> MKIQMRNKKVLSFLTLTAIVSQALVYPVYAQTSTSNHSNKKKEIVNEDILPNNGLMGYYFTDEHFKDLKLMAPIKDGNLKFEEKKVDKLLDKDKSDVKSIRWTGRIIPSKDGEYTLSTDRDDVLMQVNTESTISNTLKVNMKKGKEYKVRIELQDKNLGSIDNLSSPNLYWELDGMKKIIPEENLFLRDYSNIEKDDPFIPNNNFFDPKLMSDWEDEDLDTDNDNIPDSYERNGYTIKDLIAVKWEDSFAEQGYKKYVSNYLESNTAGDPYTDYEKASGSFDKAIKTEARDPLVAAYPIVGVGMEKLIISTNEHASTDQGKTVSRATTNSKTESNTAGVSVNVGYQNGFTANVTTNYSHTTDNSTAVQDSNGESWNTGLSINKGESAYINANVRYYNTGTAPMYKVTPTTNLVLDGDTLSTIKAQENQIGNNLSPGDTYPKKGLSPLALNTMDQFSSRLIPINYDQLKKLDAGKQIKLETTQVSGNFGTKNSSGQIVTEGNSWSDYISQIDSISASIILDTENESYERRVTAKNLQDPEDKTPELTIGEAIEKAFGATKKDGLLYFNDIPIDESCVELIFDDNTANKIKDSLKTLSDKKIYNVKLERGMNILIKTPTYFTNFDDYNNYPSTWSNVNTTNQDGLQGSANKLNGETKIKIPMSELKPYKRYVFSGYSKDPLTSNSIIVKIKAKEEKTDYLVPEQGYTKFSYEFETTEKDSSNIEITLIGSGTTYLDNLSITELNSTPEILDEPEVKIPTDQEIMDAHKIYFADLNFNPSTGNTYINGMYFAPTQTNKEALDYIQKYRVEATLQYSGFKDIGTKDKEMRNYLGDPNQPKTNYVNL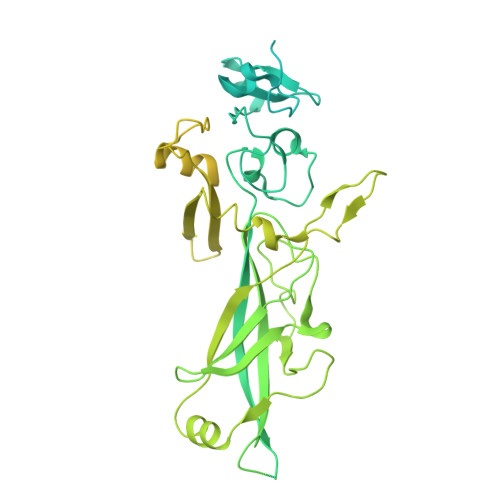RSYFTGGENIMTYKKLRIYAITPDDRELLVLSVD>[2x]GTGRSRLLEDFRNN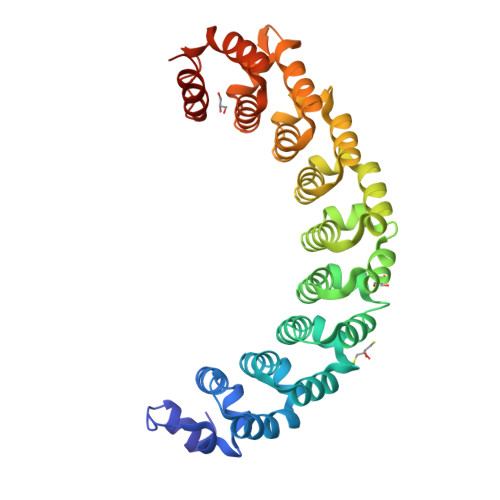RFPNLQLRDLIGHIVEFSQDQHGSRFIQQKLERATPAERQIVFNEILQAAYQLMTDVFGNYVIQKFFEFGSLDQKLALATRIRGHVLPLALQMYGCRVIQKALESISSDQQSEMVKELDGHVLKCVKDQNGNHVVQKCIECVQPQSLQFIIDAFKGQVFVLSTHPYGCRVIQRILEHCTAEQTLPILEELHQHTEQLVQDQYGNYVIQHVLEHGRPEDKSKIVSEIRGKVLALSQHKFASNVVEKCVTHASRAERALLIDEVCCQNDGPHSALYTMMKDQYANYVVQKMIDMAEPAQRKIIMHKIRPHITTLRKYTYGKHILAKLEKYYLKNSPDLG>SYLGSEFDNVELKDLANVLSFGEAKLGDNGQKFNFLFHTASSNVWVPSIKCTSESCESKNHYDSSKSKTYEKDDTPVKLTSKAGTISGIFSKDLVTIGKLSVPYKFIEMTEIVGFEPFYSESDVDGVFGLGWKDLSIGSIDPYIVELKTQNKIEQAVYSIYLPPENKNKGYLTIGGIEERFFDGPLNYEKLNHDLMWQVDLDVHFGNVSSKKANVILDSATSVITVPTEFFNQFVESASVFKVPFLSLYVTTCGNTKLPTLEYRSPNKVYTLEPKQYLEPLENIFSALCMLNIVPIDLEKNTFVLGDPFMRK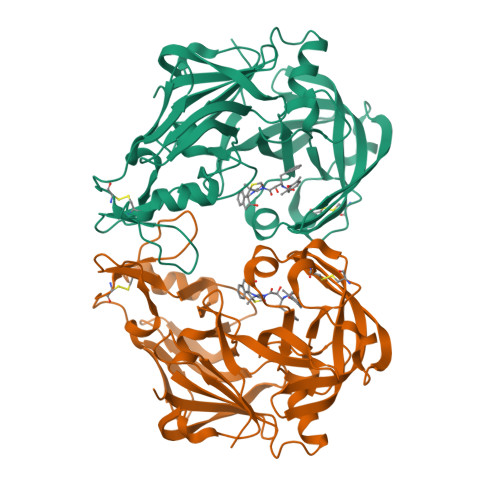YFTVYDYDNHTVGFALAKNL[4x]> MFLFFFCDLFWLRLLLCMYYCVWSRLCFIVYFNCLMLIFDFLLFCLFDLYLFVGLCLFLLLWFMLFNLYSLILYYCITYLNLYLLFCIVFLLYIAFLFLFCFLCDFFLFNNLLVGDSFMDVFFIRFLLCFLECFSLLCRCLSTFLRLFCNLLSSHFLLLMFFDFFYFIFVFFFYGVFCYWFILFIFVFCFCLLFYVF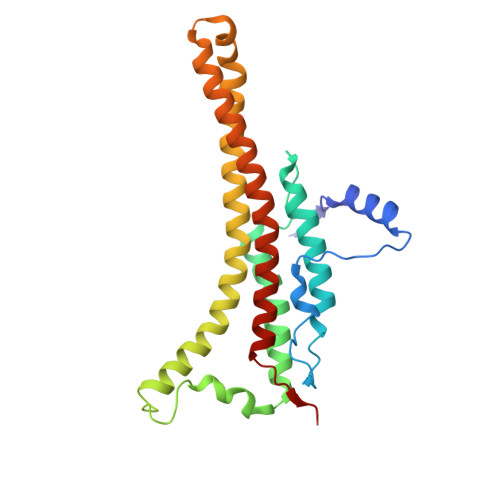LYLLDLFAAILQLFIFCNMILQLIMDFLLFLLFV> HPYYLRSFLVVLKTVLENEDDMLLFDEQEKGIVTKFYQLSATGQKLYVRLFQRKLSWIKMTKLEYEEIALDLTPVIEELTNAGFLQTESELQELSEVLELLSAPELKSLAKTFHLVNPNGQKQQLVDAFLKLAKQRSVCTWGKNKPGIGAVILKRAKALAGQSVRICKGPRAVFSRILLLFSLTDSMEDEDAACGGQGQLSTVLLVNLGRMEFPSYTINRKTHIFQDRDDLIRYAAATHMLSDISSAMANGNWEEAKELAQCAKRDWNRLKNHPSLRCHEDLPLFLRCFTVGWIYTRILSRFVEILQRLHMYEEAVRELESLLSQRIYCPDSRGRWWDRLALNLHQHLKRLEPTIKCITEGLADPEVRTGHRLSLYQRA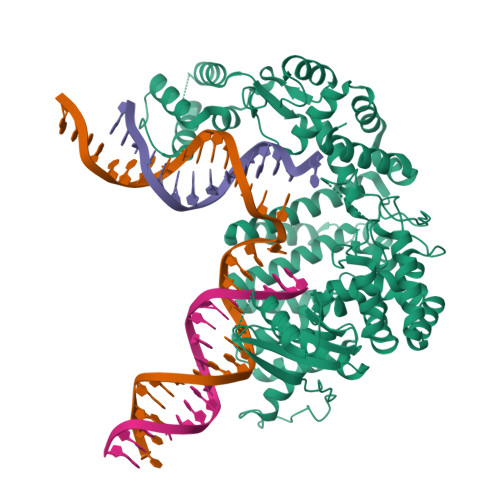VRLRESPSCKKFKHLFQQLPEMAVQDVKHVTITGRLCPQRGMCKSVFVMEAGEAADPTTVLCSVEELALAHYRRSGFDQGIHGEGSTFSTLYGLLLWDIIFMDGIPDVFRNACQAFPLDLCTDSFFTSRRPALEARLQLIHDAPEESLRAWVAATWHEQEGRVASLVSWDRFTSLQQAQDLVSCLGGPVLSGVCRHLAADFRHCRGGLPDLVVWNSQSRHFKLVEVKGPNDRLSHKQMIWLAELQKLGAEVEVCHVV> QFAKPEDAVKYRQSAFTLMASHFGRMTPVVKGQAPYDAAQIKANVEVLKTLSALPWAAFGPGTEGGDARPEIWSDAASFKQKQQAFQDNIVKLSAAADAGDLDKLRAAFGDVGASCKACH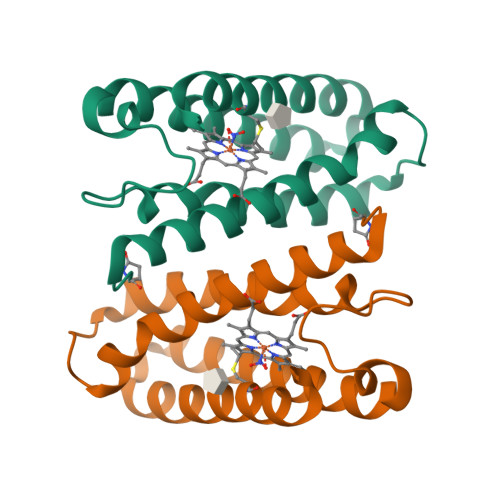DAYRK>GHMACDGLARQPEEVVLQASVSSYHLFRDVAEVTAFRGSLLSWYDQEKRDLPWRRRAEDEMDLDRRAYAVWVSEVMLQQTQVATVINYYTGWMQKWPTLQDLASASLEEVNQLWAGLGYYSRGRRLQEGARKVVEELGGHMPRTAETLQQLLPGVGRYTAGAIASIAFGQATGVVDGNVARVLCRVRAIGADPSSTLVSQQLWGLAQQLVDPARPGDFNQAAMELGATVCTPQRPLCSQCPVESLCRARQRVEQEQLLASGSLSGSPDVEECAPNTGQCHLCLPPSEPWDQTLGVVNFPRKASRKPPREESSATCVLEQPGALGAQILLVQRPNSGLLAGLWEFPSVTWEPSEQLQRKALLQELQRWAGPLPATHLRHLGEVVHTFSHIKLTYQVYGLALEGQTPVTTVPPGARWLTQEEFHTAAVSTAMKKVFRVYQGQQPGTCMGSKRSQVSSPCSR[2x]

MUTYH is a clinically important DNA glycosylase that thwarts mutations by initiating base-excision repair at 8-oxoguanine (OG):A lesions. Improperly placed adenines within pro-mutagenic OG:A base pairs are removed by the adenine glycosylase MUTYH, as the first step in Base Excision Repair (BER). The [4Fe-4S] cluster is coordinated by four cysteine ligands within the N-terminal catalytic domain, while the Zn(II) ion is coordinated by three cysteine ligands in the interdomain connector region (IDC) and one histidine within the catalytic domain. A loop made by two Cys residues that coordinate the [4Fe-4S] cluster, referred to as the iron-sulfur cluster loop, mediates electrostatic interactions with the DNA backbone that are critical for recognition of the lesion containing substrate.

To provide insight into the impact of cancer associated variants (CAVs) and roles of the [4Fe-4S] cofactor in MUTYH function, we obtained the first crystal structure of human MUTYH in complex with DNA and defined structure-function relationships for 12 [4Fe-4S] associated CAVs. Crystals diffracted to high resolution (1.9 Å) with a synchrotron source and refinement yielded final R/Rfree values of 0.180/0.209. In the MUTYH-TSAC, MUTYH embraces the entire DNA helix with contacts mediated by the two functional domains in a manner similar to other MutY homologs. However, within the IDC region we were unable to observe electron density for residues 324-347 in chain A and 319-346 in chain D (there are two copies of the MUTYH-TSAC in the asymmetric unit) nor did we observe electron density for the Zn and its coordination sphere. X-ray absorption spectra of the MUTYH-TSAC crystals lacked the ~9650-eV peak characteristic for Zn. These observations suggest Zn was lost during the crystallization process. Intriguingly, inspection of the MUTYH-TSAC crystal structure revealed an intricate hydrogen bonding network that spans the 20 Å distance between the [4Fe-4S] cluster and the adenine excision pocket. The connection involves four residues with strong evolutionary signals as shown by residue coupling correlation analysis, starting with the [4Fe-4S] cluster ligand Cys290 that H-bonds with Arg241, which in turn interacts with Asn238, and lastly this Asn residue H-bonds with the key catalytic residue Asp236. In addition, the amide hydrogen of the side chain of the Asn238 also interacts with the 5’ phosphate of the 1N nucleotide. These connections make use of the multivalent Arg241 and Asn238 residues: Arg241 adopts a C-like shape that enables the positioning of internal NH1ε moiety of the guanidine group to donate a H-bond to the main chain carbonyl amide of Cys290.>MSKYERPLKRESQIKEFELGTHAAVIEKVQKKRSQKGNDMFLLSLLGKSNEKGVYFLTFGNDYTEDNLRYILASIQDNGVEIPDVDFGYNRETFEFLKGKDVYIQVEEQEYKGKVKHAVTNFLTQDEFEESEEMEFSESNTEEDW[3x]

Here, we characterize PrgE, a proposed SSB from the Enterococcus faecalis plasmid pCF10. Structurally, it has the characteristic OB-fold of SSBs, but it has very unusual DNA-binding properties. Unlike other SSBs, PrgE binds both double- and single-stranded DNA equally well. This shows that PrgE has a quaternary assembly and DNA-binding properties that are very different from the prototypical bacterial SSB, but also different from eukaryotic SSBs.

We also crystallized PrgE together with a single-stranded poly-A 60-mer DNA in a molar ratio of 1:3. The obtained crystallographic data were refined in the space group P212121 with the asymmetric unit containing three copies of the protein sitting on a string of 15 ssDNA bases. Although there are only 15 bases in the asymmetric unit, the ssDNA shows a continuous density throughout the crystal packing. Compared with the apo structure of PrgE, a few more residues are visible at the C-terminal end (until residues 136 of 144), continuing as an alpha-helix as predicted by the AlphaFold2 model. The DNA does not get wrapped around PrgE, like it does with E. coli SSB; rather, PrgE interacts with the DNA like beads on a string, with the N-terminal tail of one PrgE binding to the neighboring PrgE, using interactions between polar side chains. PrgE binds to the ssDNA between loops 1 and 4, where the beta-barrel is partially open. Each subunit binds to five DNA bases. The binding also bends the ssDNA between the protein-binding sites, resulting in a kink at every fifth base. Many interactions with the phosphate backbone of the ssDNA are the same within all subunits, including with residues Ser33, Gln34, and Asn37 in loop 1 that form H-bonds with the DNA backbone with the fourth and fifth phosphate of each stretch of five bases. In addition to hydrogen bonding with the phosphate backbone, pi–pi interactions between the aromatic rings of the DNA and two tyrosine residues are of major importance for DNA binding.> MGELVRTDSPNFLCSVLPTHWRCNKTLPIAFKVVAK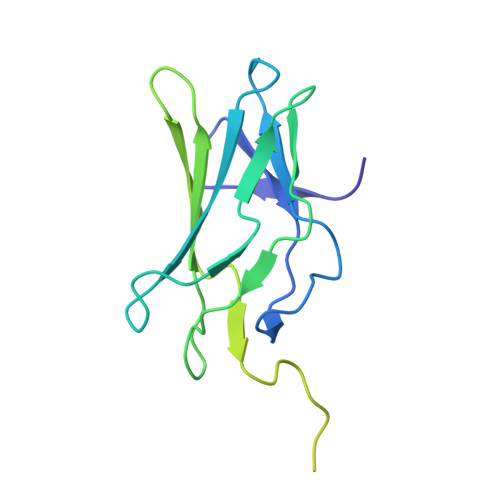GDVPDGTLVTVMAGNDENYSAELRNATAAMKNQVARFNDLRFVGRSGRGKSFTLTITVFTNPPQVATYHRAIKITVDGPREPRRHRQKLDDQTKPGSLSFSERLSELEQLRRTAMRVSPHHPAPTPNPRASLNHSTAFNPQPQSQMQDARQIQPSPPWSYDQSYQYLGS5-chloro-1H-indole | C8 H6 Cl N | 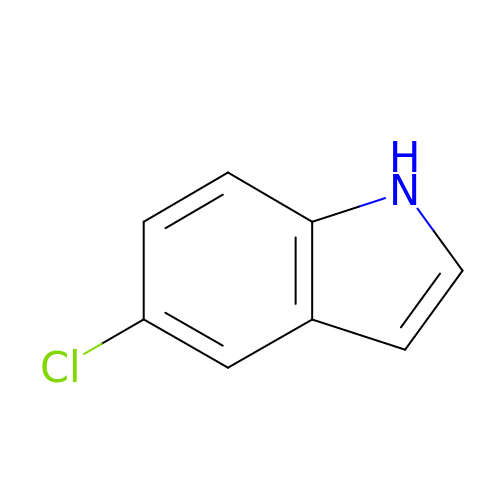MYTGFBZJLDLWQG-UHFFFAOYSA-N> HMERPESELIRQSWRVVSRSPLEHGTVLFARLFALEPSLLPLFQGGGQFSS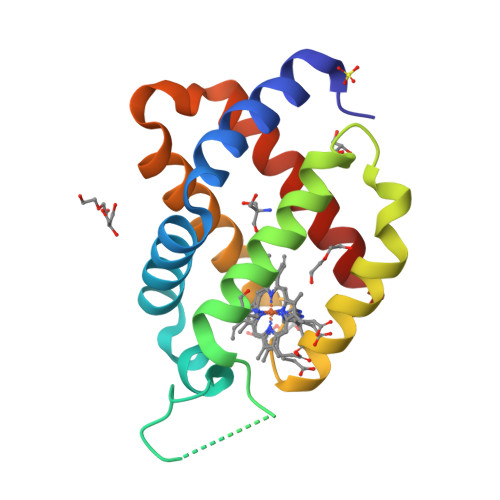PEDSLSSPEFLDHIRKVMLVIDAAVTNVEDLSSLEEYLTSLGRKHRAVGVRLSSASTVGESLLYMLEKSLGPDFTPATRTAWSRLYGAVVQAMSRGW>[2x]MKRVVITGMGIISSIGNNVEEVLASLKAGKSGITASEQFKEHGLRSQVWGDLKINPEEHIDRKQMRFMGDAAAYAYLSLEQAIADAGLTPEQVSNDRTGIVAGSGGASSENQVIAVDTQREKGVKRVG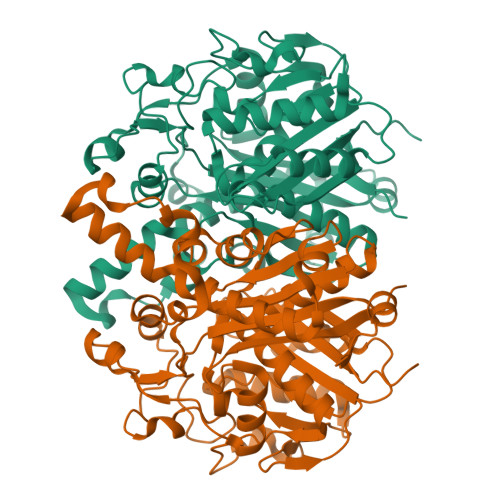PYMVPRTMSSTVSACLATPFKIRGVNYSISSACATSAHCIGNAVELIQLGKQDIVFAGGGEELYWSQTMMFDAMGALSTKYNETPEKASRTYDADRDGFVISGGGGMVVVEELEHALARGAKIYGEIVGYGATSDGYDMVAPSGEGAIRCMKMAMQGVDKIDYINTHGTSTPVGDVKELGAIQEVFGGNSPAISATKAMTGHALGAAGVHEAIYSTLMLHHGFIAPSINIDTLDEAAQGLDIVTELREQELTTVMSNSFGFGGTNATLVIKKYQGL>[3x]MTTKKADYIWFNGEMVRWEDAKVHVMSHALHYGTSV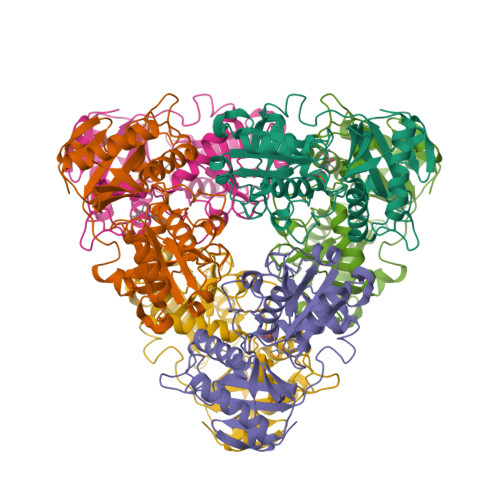FEGIRCYDSHKGPVVFRHREHMQRLHDSAKIYRFPVSQSIDELMEACRDVIRKNNLTSAYIRPLIFVGDVGMGVNPPAGYSTDVIIAAFPWGAYLGAEALEQGIDAMVSSWNRAAPNTIPTAAKAGGNYLSSLLVGSEARRHGYQEGIALDVNGYISEGAGENLFEVKDGVLFTPPFTSSALPGITRDAIIKLAKELGIEVREQVLSRESLYLADEVFMSGTAAEITPVRSVDGIQVGEGRCGPVTKRIQQAFFGLFTGETEDKWGWLDQVNQ> SYSTLANFPVQARNDNISPWTITGFADAESSFMLTVSKDSKRNTGWSVRPRFRIGLHNKDVTILKSIREYLGAGIITSDIDARIRFESLK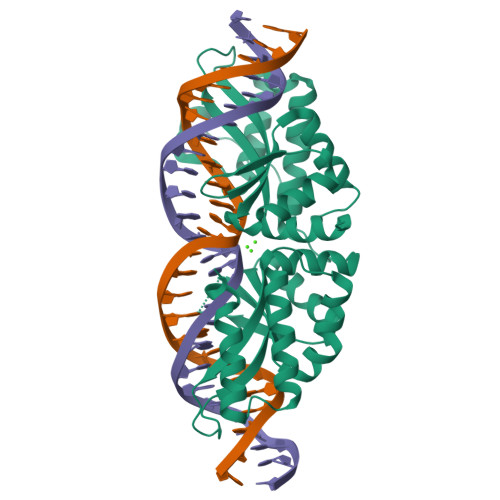ELEVVINHFDKYPLITQKRADYLLFKKAFYLIKNKEHLTEEGLNQILTLKASLNLGLSEELKEAFPNTIPAERLLVTGQEIPDSNWVAGFTAGDGSFYIRIAKNSTLKTGYQVQSVFQITQDTRDIELMKNLISYLNCGNIRIRKYKGSEGIHDTCVDLVVTNLNDIKEKIIPFFNKNHIIGVKLQDYRDWCKVVTLIDNKEHLTSEGLEKIQKIKEGMNRGRSL>[2x]SLFELGKMILQETGKNP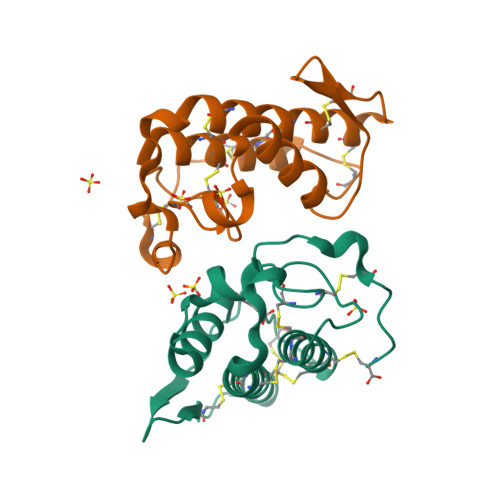AKSYGVYGCNCGVGGRGKPKDATDRCCYVHKCCYKKLTGCDPKKDRYSYSWKDKTIVCGENNSCLKELCECDKAVAICLRENLDTYNKKYRYNYLKPACKKADPC> MLKAWHLPVAPFIKEQQERLMITLWLSGDDLPPRVTLRAEEDNEELSLPMHRLRQAPHPGVVAWRGEINLVNGQPRRRYSFKLLWADRQLWFTPQEFNRFPPARLEQFAV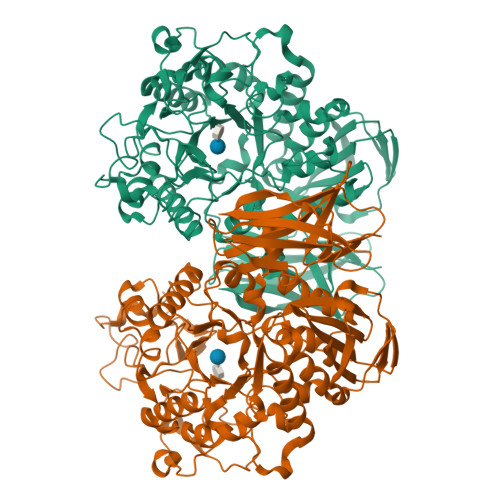DLPDSGPQWVADQVFYQIFPDRFARSQSREAEQDATYYHHAAGHDIVRKAWDEPLTAEAGGSTFYGGDLDGISEKLPYLKQLGVTALYLNPVFVAPSVHKYDTEDYRRVDPQFGGDAALLRLRHNTQKEGMRLILDGVFNHSGDSHAWFDRHQRGSGGACHNADSPWRDWYNFSPEGVAHDWLGYASLPKLDYRSSTLIDEIYGGEDSVVRHWLKAPWSMDGWRLAVVHMLGEGGGARNNLRHIAGITQAAKLERPDAFVFGEHFGDARQWLQADVEDSAMNYRGFTFPLWGFLANTDISYDPQKIDAQTCMAWMDNYRAGLSHQQQLRMFNQLDSHDTARFKSLLGKDVARLPLAVVWLFSWPGVPCIYYGDEVGVDGNNDPFCRKPFPWDPALQDGDLLDLYKRMSKLRKAHQALRYGGCQVIYAEDNVVVFVRVYKQQRVLVAINRGEACEVVIEDSPLLDVNGWQLKEGAGALHDGVLTLPAISASVWFSR> MIDKSAFVHPTAIVEEGASIGANAHIGPFCIVGPHVEIGEGTVLKSHVVVNGHTKIGRDNEIYQFASIGEVNQDLKYAGEPTRVEIGDRNRIRESVTIHRGTVQGGGLTKVGSDNLLMINAHIAHDCTVGNRCILANNATLAGHVSVDDFAIIGGMTAVHQFCIIGAHVMVGGCSGVAQDVPPYVIAQGNHATPFGV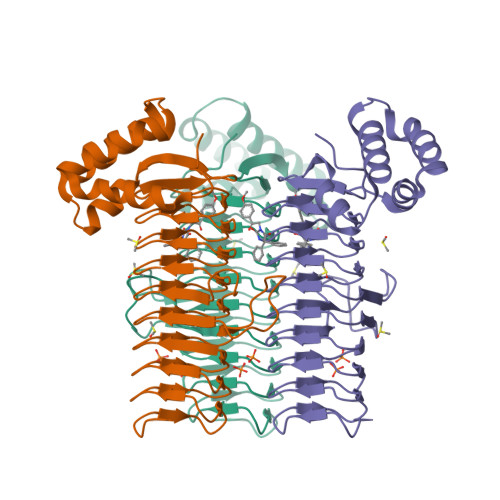NIEGLKRRGFSREAITAIRNAYKLIYRSGKTLDEVKPEIAELAETYPEVKAFTDFFARSTRGLIRHHHHHH> AYVEIIEQPKQRGMRFRYKCEGRSAGSIPGERSTDTTKTHPTIKINGYTGPGTVRISLVTKDPPHRPHPHELVGKDCRDGYYEADLCPDRSIHSFQNLGIQCVKKRDLEQAISQRIQTNNNPFHVPIEEQRGDYDLNAVRLCFQVTV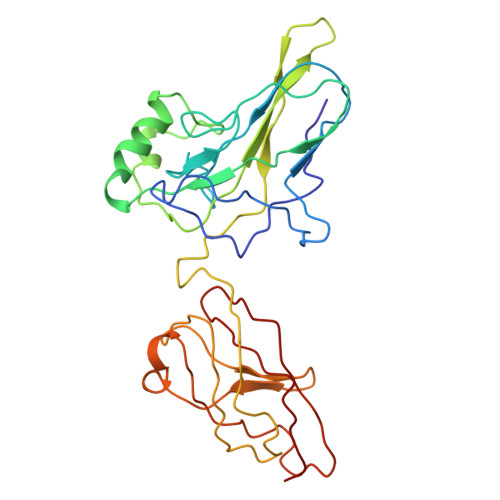RDPAGRPLLLTPVLSHPIFDNRAPNTAELKICRVNRNSGSCLGGDEIFLLCDKVQKEDIEVYFTGPGWEARGSFSQADVHRQVAIVFRTPPYADPSLQAPVRVSMQLRRPSDRELSEPMEFQYLPD>[4x]MKKLLNTLYVTQPDTYLSLDGDNVVLLKEQEKLGRLPLHNLEAIVGFGYTGASPALMGYCAERNISITFLTKNGRFLARVVGESRGNVVLRKTQYRISENDQESTKIARNFITGKVYNSKWMLERMTREHPLRVNVEQFKATSQLLSVMMQEIRNCDSLESLRGWEGQAAINYNKVFDQMILQQKEEFAFHGRSRRPPKDNVNAMLSFAYTLLANDVAAALETVGLDAYVGFMHQDRPGRASLALDLMEELRGLYADRFVLSLINRKEMTADGFYKKENGAVLMTDEARKTFLKAWQTKKQEKITHPYLGEKMSWGLVPYVQALLLARFLRGDLDEYPPFLWK;>GSMLVLITYDVQTSSMGGTKRLRKVAKACQNYGQRVQNSVFECIVDSTQLTSLKLELTSLIDEEKDSLRIYRLGNNYKTKVEHIGAKPSIDLEDPL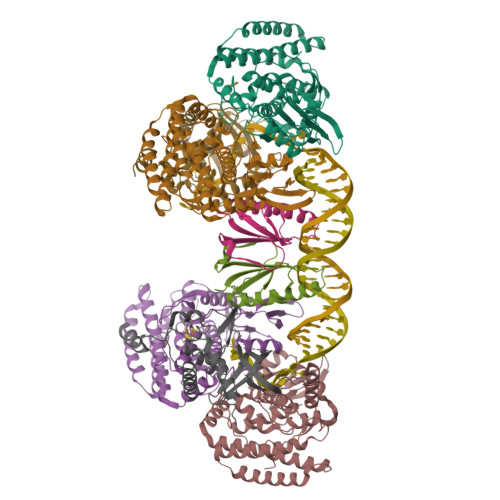IF[2x];>ASNEEDRYLMLSGLQHFQFCKRQWALIHIEQQWEENVRTIEGQHLHKKADQPFMKEKRGSKLTVRAMPIQSKNLQISGICDVVEFVQDSEGIELSGVSGSYKAFPVEYKRGKPKKGDEDIVQLVAQAMCLEEMLVCRIDKGYLFYNEIKHRVEVPITDALRDKVVQMAKEMHHYYENRHTPKVKTGPFCNNCSLQSICLPKLMNKRSVKRYIEGRLSE[2x]4-[(2R)-2-aminopropyl]phenol | C9 H13 N O | 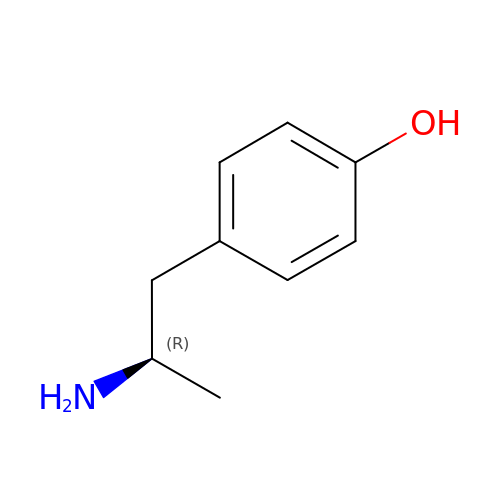GIKNHHRFLCDOEU-SSDOTTSWSA-N>GSPVVVGSKPAQRFAVLYGTMCDILNGYDNQVVMQQKLKEFIEVLRDPKLPYSEFSAQFSALHARMPHKLDAQLTQVLERAQNRGAEFPARQLLKVFNKFLDDNVPNKTDQDLLKSTLEPLTSVLNLYLDGQKARELNLIADLLSMYADVECQFSGRRLQDEEAILKLRDQYKDNIQKVVNTVLSHKNVMSKNSLVLALLDEYRPNKPNVGNVGKHLRPVLRRLTELESRQSAKVSLKAREVLILCALPSLEERTAQMEHILRSSVVQSRYGETGWSHRRPDREVLKEVVDSKYTVFDVLTLFFAHEDPYVALAALEVYVRRAYRAYNLREVRYHDEERPYFIDWDFALRKSGANQTESSMHMQSVVPSSPATPVENDFKRIHSISDMTYLARRTRDEPIRKGVIVPCKDLLDAEEALSRALEVLPLAHKETKDKDRKQQPGIAADLAQRRRPGTPLRLEGIGELSAVVNVAVRDAEGKNDEEILALIKPWVQNSKADLLARRVRRLTFICGRNDGSYPSYYTFRGPDYAEDDSIRHIEPSLAFQLELGRLSKFKLTPVFTQNKNIHVYEAVGRGVETDRRYFTRAVVRPGRLRDEISTAEYLISEADRVVNDIFDALEIIGTNKTDLNHMFINFSHTFQVTADEVAESLQGFLDRFGPRGWRLRVHQVEIRINCMRSDNNDENDTMPLRVIITNTSGFVIQIELYEEKLSEKGEWVYYYVSGNAKIGSMHLLPVSTPYPTKNWLQPKRYKAHILGTQYVYDFPELFRQAIQNSWTEAVKKIPSLAAKQPAIGECIDYNELVLGDQDNLAEVSREPGMNSTGMVGWLINARTPEYPDGRKFIVVANDITFKIGSFGPKEDTFFFKCTELARKMGIPRIYLSANSGARLGLAEELMPHFNVAWNDPAKPEAGFKYLYLSDEAKRRFENEVITEEIVEDGEKRHKIITIVGAEEGLGVECLRGSGLIAGATSRAYNDIFTCTLVTCRSVGIGAYLVRLGQRAVQVEGQPIILTGAPALNSLLGREVYTSNLQLGGTQIMYRNGVSHLTAKDDFDGVTKIVQWLSFIPDQRNNPLPILSPSPDPWDRDVVYTPPYKQTYDVRWMIAGKEDEDGFQPGLFDKDSFVETLGGWARTVVVGRARLGGIPMGVIAVETRTIENITPADPANPDSIEQVTNEAGGVWYPNSAFKTAQAINDFNYGEQLPLMILANWRGFSGGQRDMYNEVLKYGSFIVDALTRFEKPIFIYIPPHGELRGGSWVVVDPTINPASMEMYADEEARGGVLEPEGIIPIKYKKDKQLETMARLDPVYRSLKKEMAKEGLSKEESDNIKKKMQQREELLLPIYHQICVQFADLHDRAGRMKAKGVIRQSLQWRQSRRFFYWRVRRRLIEDDILRRIEEAINPAGKRRHDPENTSLAASPETRSPHLVQLESWVGIPGFKTNDREVVEWYEQNQDRINEKLEKLKKESIADQMRELLRXXXXXXXXXXXX[2x]

Biotin-dependent acetyl-CoA carboxylases (ACCs) are essential enzymes that catalyse the ATP-dependent carboxylation of acetyl-CoA to malonyl-CoA. Eukaryotic ACCs, instead, are multienzymes, which integrate all functional components into a single polypeptide chain of ∼2,300 amino acids2. In addition to the canonical ACC components, eukaryotic ACCs contain two non-catalytic regions, the large central domain (CD) and the BC–CT interaction domain (BT). Here we provide the structure of Saccharomyces cerevisiae (Sce) ACC CD, intermediate- and low-resolution structures of human (Hsa) ACC CD and larger fragments of fungal ACC from Chaetomium thermophilum (Cth).

Using molecular replacement based on fungal ACC CD and CT models, we obtained structures of a variant comprising CthCT and CDC1/CDC2 in two crystal forms at resolutions of 3.6 and 4.5 Å (CthCD-CTCter1/2), respectively, as well as of a CthCT linked to the entire CD at 7.2 Å resolution (CthCD-CT). Owing to the limited resolution the discussion of structures of CthCD-CT and CthΔBCCP is restricted to the analysis of domain localization. In all these crystal structures, the CT domains build a canonical head-to-tail dimer29, with active sites formed by contributions from both protomers. However, MS analysis of CthCD-CT and CthΔBCCP constructs revealed between 60 and 70% phosphorylation of Ser1170 (corresponding to SceACC Ser1157). The CDN domain positioning relative to CDL/CDC1 is highly variable with three main orientations observed in the structures of SceCD and the larger CthACC fragments: CDN tilts, resulting in a displacement of its N terminus by 23 Å (observed in both protomers of CthCD-CT and one protomer of CthΔBCCP, denoted as CthCD-CT1/2 and CthΔBCCP1, respectively). The CDC2/CT interface acts as a true hinge with observed rotation up to 16°, which results in a translocation of the distal end of CDC2 by 8 Å. The interface between CDC2 and CDL/CDC1, which is mediated by the phosphorylated regulatory loop in the SceCD structure, is less variable than the CD–CT junction, and permits only limited rotation and tilting. Analysis of the impact of phosphorylation on the interface between CDC2 and CDL/CDC1 in CthACC variant structures is precluded by the limited crystallographic resolution.> LKTEWPELVGKSVEEAKKVILQDKPEAQIIVLPVGTIVTMEYRIDRVRLFVDKLDNIAEVPRVG

As scaffold for implementing fold-switched allosteric assemblies, we chose chymotrypsin inhibitor 2 (CI2) from barley seeds. The small (<70 residues) globular single-domain CI2 is a paradigm of two-state folding in which a sturdy native structure unfolds at an extremely slow rate via an all-or-none transition. The CI2 native structure contains a four-stranded β-sheet and one α-helix connecting strands 1 and 2. The C-terminal β-strand is inserted in antiparallel fashion into the sheet’s middle, breaking an otherwise parallel arrangement to form a unique fold that is specific to this family of serine protease inhibitors.

To identify possible spatial arrangements for assembly, we analyzed the crystal lattice of CI2 by X-ray crystallography. CI2 crystallizes in the hexagonal space group P622 in all the conditions we attempted that rendered crystals. On the lattice, the protein forms double hexameric rings in which the two rings are packed head to head and rotated by ~30°. This spatial arrangement is strongly predefined by symmetry, and thus we identify the toroidal D6 particles of the crystal as the target for engineering a CI2 assembly. An unexpected discovery was that we observed domain swapping at certain crystallization conditions. Indeed, crystals obtained using salt as primary precipitant follow the standard arrangement of early structural work on CI241 (left), whereas crystals grown with PEG feature domain-swapped dimers arranged in the same lattice structure and group symmetry (right). In domain-swapped crystals, equivalent monomers on the two rings exchange their C-terminal segments (residues 39–66) to form dimers that covalently link the rings via the active loops (right). Domain swapping does not affect the monomer–monomer interface of each ring, and thus is unable to self-sufficiently promote assembly in solution, but it does demonstrate an inherent tendency of the C terminus of CI2 to unwind, and the robustness of the toroidal D6 packing symmetry for this protein.First isolated in 1991 from the fungus identified as Paecilomyces variotii SANK 21086, cornexistin (6) was shown to display excellent post‐emergence efficacy against a range of weed species, whilst also exhibiting selectivity for corn. Because of its unique chemical structure and its promising weed control profile, cornexistin (6) has been the topic of several research programs over the years. This has included the MoA elucidation of cornexistin (6), i. e., its capacity at inhibiting transketolase (TK; EC.2.2.1.1) [11f] which is an important enzyme in both the Calvin‐Benson‐Bassham cycle and the oxidative pentose phosphate pathway in chloroplasts. In TK, the TPP cofactor is bound in a deep cleft at the interface of the monomers in the dimeric enzyme. Guided by an X‐Ray co‐crystal structure of cornexistin bound to transketolase from Zea mays, we attempted to identify the key interactions that are necessary for cornexistin to maintain its herbicidal profile.

To better understand the molecular basis of cornexistin binding to its target enzyme, we determined the X‐ray crystal structure of cornexistin in complex with TK from Zea mays at a resolution of 1.9 Å. The X‐ray co‐crystal structure reveals that cornexistin binds to residues from both TK monomers in its diacid form 7 (presumably arising from hydrolysis of the maleic anhydride) thus effectively blocking the entrance to the TK active site. The two carboxyl groups of diacid 7 interact with the sidechains from Arg369, Ser396, His474 and Arg533 of the first monomer. In addition, hydrogen bonds are observed from the C2‐hydroxyl group to the sidechain of Asp482 from the same monomer and from the C8‐hydroxyl group to mainchain atoms from Gly37 and Gly276 of the second monomer. It should be noted that the shortest distance between the atoms from diacid 7 and the TPP cofactor in the crystal structure is 6.6 Å, effectively showing that they are not interacting with each other when engaging TK. Further examination of the C1‐carbonyl group determined that there was no direct hydrogen bond formation with the TK protein, instead it interacts with the protein via a network of tetrahedrally coordinated water molecules. The importance of the C2‐hydroxyl group close to the alkyl moiety was then explored. This hydroxyl group bridges directly to the sidechain of Asp482B and via an internal water molecule to the side chain of His38A. Lastly, closer investigation of the C3‐propyl side chain revealed that it provides significant stabilization via the hydrophobic effect, since the side chain is buried in a hydrophobic pocket of the protein‐protein interface. We confirmed Zea mays TK inhibition in the double‐digit μM‐range (IC50=50±5 μM). In contrast, the C2‐hydroxyl group is prominently involved in a hydrogen bonding network to Asp482 from the first monomer and two adjacent water molecules that in turn are near the reactive ylide of the TPP cofactor.

>MHHHHHHENLYFQGAVETLQGKAATGELLEKSVNTIRFLAIDAVEKANSGHPGLPMGCAPMGHVLYDEVMRYNPKNPYWFNRDRFVLSAGHGCMLQYALLHLAGYDSVKEEDLKQFRQWGSRTPGHPENFETPGVEVTTGPLGQGIANAVGLALAEKHLAARFNKPDSEIVDHYTYVILGDGCQMEGIANEACSLAGHWGLGKLIAFYDDNHISIDGDTEIAFTEDVSTRFEALGWHTIWVKNGNTGYDDIRAAIKEAKAVTDKPTLIKVTTTIGFGSPNKANSYSVHGSALGAKEVEATRQNLGWPYDTFFVPEDVKSHWSRHTPEGAALEADWNAKFAEYEKKYADDAATLKSIITGELPTGWVDALPKYTPESPGDATRNLSQQCLNALANVVPGLIGGSADLASSNMTLLKMFGDFQKDTAEERNVRFGVREHGMGAICNGIALHSPGFVPYCATFFVFTDYMRGAMRISALSEAGVIYVMTHDSIGLGEDGPTHQPIEHLVSFRAMPNILMLRPADGNETAGAYKVAVLNRKRPSILALSRQKLPHLPGTSIEGVEKGGYTISDNSTGNKPDLIVMGTGSELEIAAKAADELRKEGKTVRVVSFVSWELFDEQSDEYKESVLPAAVTARISIEAGSTLGWQKYVGAQGKAIGIDKFGASAPAGTIYKEYGITVESIIAAAKSF[3x]> MSPWERILLEEILSEPVRLVKERVRTHTGRELTYVYRPGPVAASFVLPVTERGTALLVRQYRHPTGKFLLEVPAGKVDEGETPEAAARRELREEVGAEAETLIPLPSFHPQPSFTAVVFHPFLALKARVVTPPTLEEGELLESLEL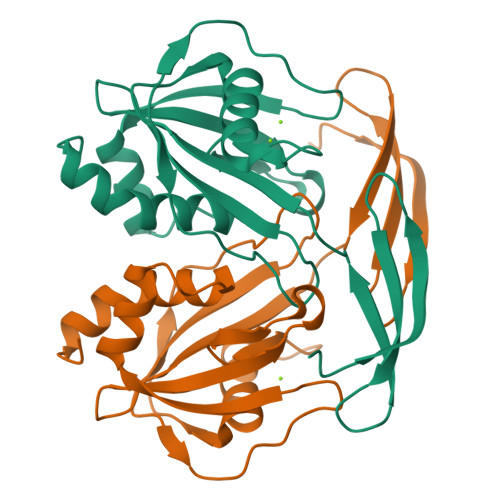PLTEVYALLAKGEIQDASTALTLFYAEPHLKRLGLL>MGHHHHHHHHHHSSGHIDDDDKHMPAHASPFNAPSSASRAGAARLGTSRRFAPFVLAALAILMGAMSVVALCVGAYRIPLAEAWAALSGDPAAQQARAVLLDIRAPRVVLALLVGGGFGATGAAMQALFRNPLADPGLVGVSSGAALGATTLIVLGPALFAAHASAAALPVAAFAGGLAVAALVYRLAASRGRLALPLLLLAGIAINALVGAAIGLLTFVADDAQLRSLTFWSLGSLGGAQWPTLAAVAPCVALGGVLLVRERDALNALQLGETEALHLGVPVQRLKRRVLVAVALAVGALVSCAGIIGFIGLVAPHCVRLACGPDQRIVLPGAALLGALLTLAADLAARTVAAPADIPLGVLTALLGAPFFLALLWKNRGALGG[2x];>[2x]MLTAHHLDVARRHGTILRDLSLSIEPGRVTALLGRNGAGKSTLLKTFAGELTGSVAPHGVRVTGDVTLNGEPLARIDAPRLACLRAVLPQAAQPAFPFSVDEIVLLGRYPHARRSGATSHRDRDIAWRALERAGADALVGRDVTTLSGGELARVQFARVLAQLWPDHDTTEPGPRYLLLDEPTAALDLAHQHRLLDTVRAVAREWQLGVLAIVHDPNLAARHADAIAMLADGTIVAHGAPRDVMTPAHIAQCYGFAVKMVETGDGTPPVMVPA;> GPLGSKRVIVIGGALAETAFALGGAETPRYRLVGADTTCTYPDAAKRLPKVGYQRALSAEGLLSLRPDLVLASAEAGPPTAIAQVKGAGVTVTTFDERHDVESVRAKITGVAQALDVRDAGAALLQRFDRDWQAARDAVAARVP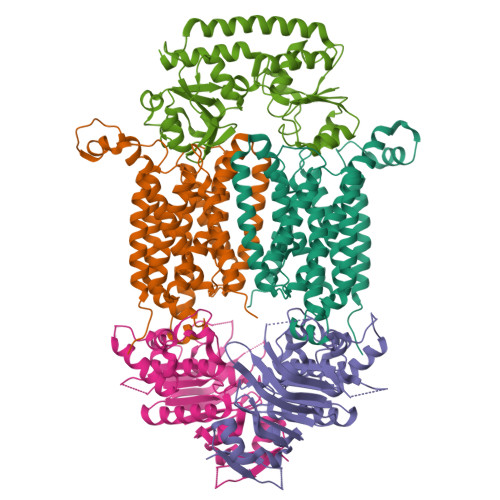GGAQPPRVLFVLNHTGTQALVAGQRTAADAMIRYAGARNAMQGFDHYKPLTTEALAAAAPDVVLISDEGLAAVGGHAALLATPGFGATPAGRARRVVSLDALFLLGFGPRLPLAVTTLHRRLSDALA>[8x]SGSGMYRNFLKRVIDILGALFLLILTSPIIIATAIFIYFKVSRDVIFTQARPGLNEKIFKIYK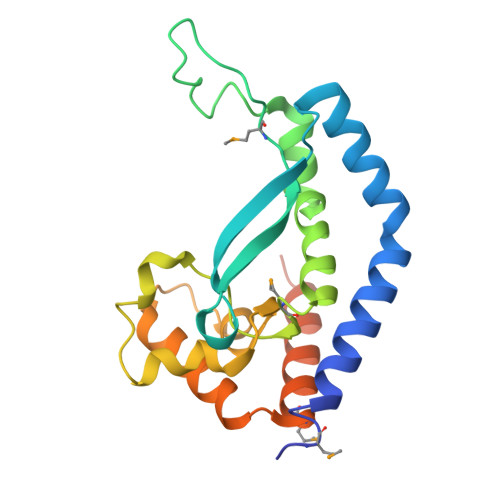FKTMSDERDANGELLPDDQRLGKFGKLIRSLSLDELPQLFNVLKGDMSFIGPRPLLVEYLPIYNETQKHRHDVRPGITGLAQVNGRNAISWEKKFEYDVYYAKNLSFMLDVKIALQTIEKVLKRSGVSKEGQATTEKFNGKN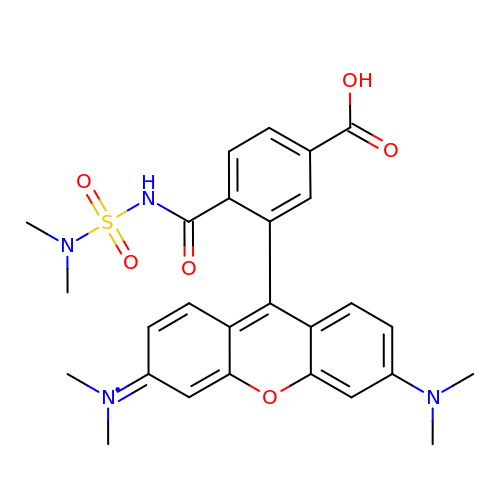3-[3-(dimethylamino)-6-(dimethyl-$l^{4}-azanylidene)xanthen-9-yl]-4-(dimethylsulfamoylcarbamoyl)benzoic acid | C27 H29 N4 O6 S | WYGUIDZIZZOQBY-UHFFFAOYSA-N6-O-phosphono-beta-D-psicofuranosonic acid | C6 H11 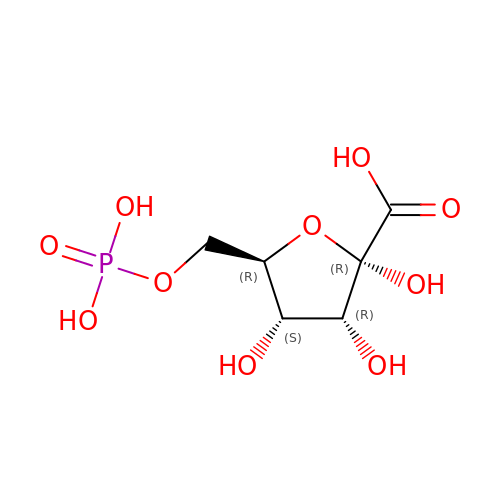O10 P | LXQWHMQOSMCJIZ-ZGEUXELVSA-N>EAASSSDADGKEVGSSGEGNRATGGKWRRPSLAQQRARRAQLPPAFDVVHWNDEDISRGHLLRVLHRDTFVVLDYHRQARMLTEEGNKAERVVSVMLPAVYTARFLAVLEGRSEKVEVHSRYTNATFTPNPAAPYTFTLKCTSTRPAQQKQQVAGEEGDETFEWTVEFDVAESLMLQRFLTQALHYNTGFARTSV[4x];>ASTFSGVQSLPKFEIHDVRDDPAEGTMTRVAVDGKLLLISQYPQLGPRKVDPNDLSPQFDADRRISVRLRHVDLAYLVGVCK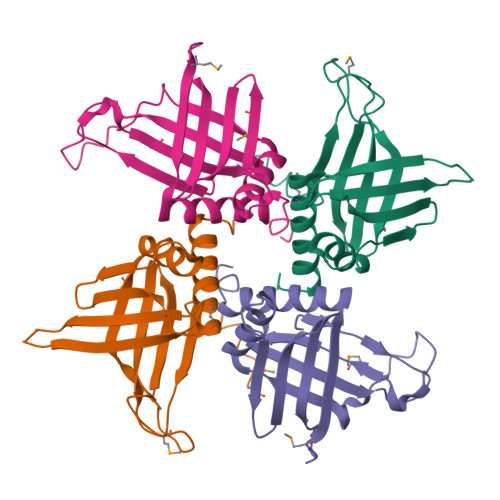ERVPRHRMETKAYTLDFEKSAQGYHLHGKVHRVASQRMEDWSVKFDNHFAVTLEHFLESALDESFGFRQHYATRAAEGGEKIAATSSAEGGARRKRSVSDTSRYH[4x]methyl (2R)-2-[(9S)-7-(4-chlorophenyl)-4,5,13-trimethyl-3-thia-1,8,11,12-tetrazatricyclo[8.3.0.0^{2,6}]trideca-2(6),4,7,10,12-pentaen-9-yl]butanoate | C22 H23 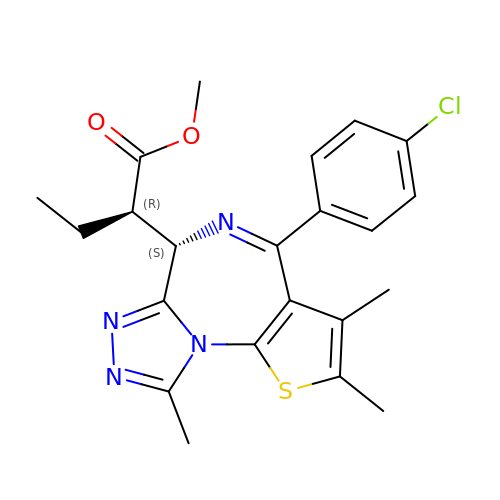Cl N4 O2 S | WLKVOOMXHSBIOW-APWZRJJASA-N6-BENZYL-1-ETHOXYMETHYL-5-ISOPROPYL URACIL | C17 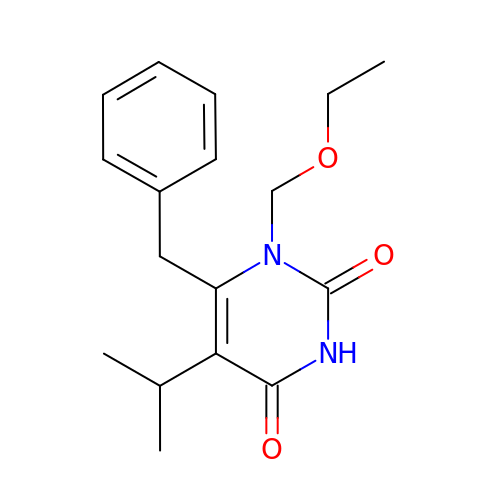H22 N2 O3 | MLILORUFDVLTSP-UHFFFAOYSA-N> 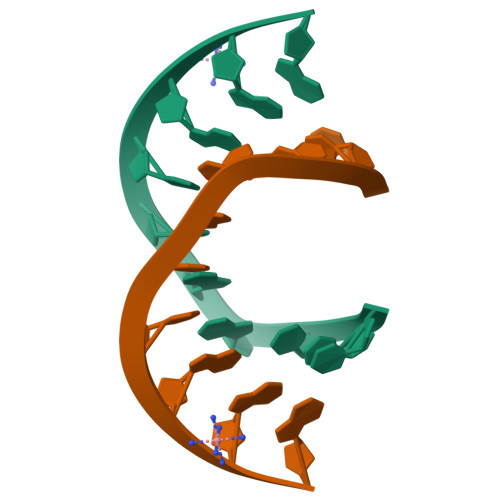CCCGATCGGG>[2x]MVPISPIETVPVKLKPGMDGPKVKQWPLTEEKIKALVEICTEMEKEGKISKIGPENPYNTPVFAIKKKDSTKWRKLVDFRELNKRTQDFWEVQLGIPHPAGLKKKKSVTVLDVGDAYFSVPLDEDFRKYTAFTIPSINNETPGIR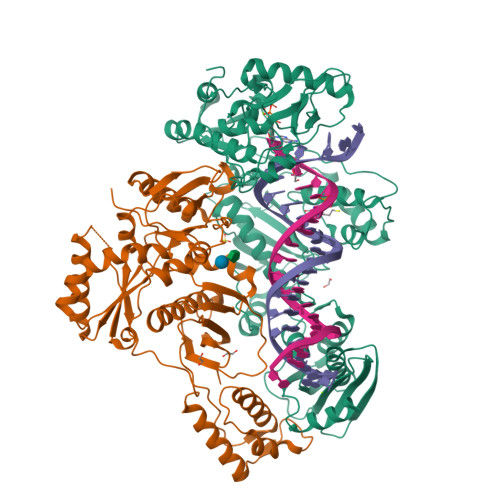YQYNVLPQGWKGSPAIFQSSMTKILEPFKKQNPDIVIYQYMDDLYVGSDLEIGQHRTKIEELRQHLLRWGLTTPDKKHQKEPPFLWMGYELHPDKWTVQPIVLPEKDSWTVNDICKLVGKLNWASQIYPGIKVRQLSKLLRGTKALTEVIPLTEEAELELAENREILKEPVHGVYYDPSKDLIAEIQKQGQGQWTYQIYQEPFKNLKTGKYARMRGAHTNDVKQLTEAVQKITTESIVIWGKTPKFKLPIQKETWETWWTEYWQATWIPEWEFVNTPPLVKLWYQLEKEPIVGAETFYVDGAANRETKLGKAGYVTNKGRQKVVPLTNTTNQKTELQAIYLALQDSGLEVNIVTNSQYALGIIQAQPDKSESELVNQIIEQLIKKEKVYLAWVPAHKGIGGNEQVDKLVSAG;>PISPIETVPVKLKPGMDGPKVKQWPLTEEKIKALVEICTEMEKEGKISKIGPENPYNTPVFAIKKKDSTKWRKLVDFRELNKRTQDFWEVQLGIPHPAGLKKKKSVTVLDVGDAYFSVPLDEDFRKYTAFTIPSINNETPGIRYQYNVLPQGWKGSPAIFQSSMTKILEPFKKQNPDIVIYQYMDDLYVGSDLEIGQHRTKIEELRQHLLRWGLTTPDKKHQKEPPFLWMGYELHPDKWTVQPIVLPEKDSWTVNDIQKLVGKLNWASQIYPGIKVRQLSKLLRGTKALTEVIPLTEEAELELAENREILKEPVHGVYYDPSKDLIAEIQKQGQGQWTYQIYQEPFKNLKTGKYARMRGAHTNDVKQLTEAVQKITTESIVIWGKTPKFKLPIQKETWETWWTEYWQATWIPEWEFVNTPPLVKLWYQ[2x]> APAAVDWRARGAVTAVKDQGQCGSCWAFSAIGNVECQWFLAGHPLTNLSEQMLVSCDKTDSGCSGGLMNNAFEWIVQENNGAVYTEDSYPYASGEG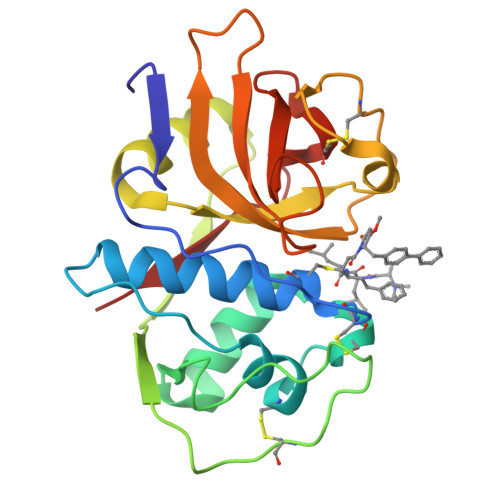ISPPCTTSGHTVGATITGHVELPQDEAQIAAWLAVNGPVAVAVDASSWMTYTGGVMTSCVSEQLDHGVLLVGYNDSAAVPYWIIKNSWTTQWGEEGYIRIAKGSNQCLVKEEASSAVVG> GGCAUCGAUCCGGCGAUCACCGGGGAGCCUUCGGAAGAACGGCCGGAAACGGCCCAGUAGAACCGAACGGGUUGGCCCGUCACAGCCUCAAGUCGAGCGGCCGCGCGAAAGCGUGGCAAGCGGGGUGGCAC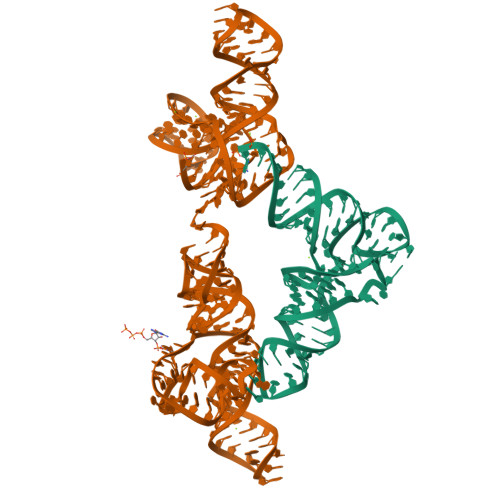CGCGGCGUUCGCGCGAAAGCGUGGCGUCGUCCCCGC;> GGGCCUAUAGCUCAGGCGGUUAGAGCGCUUCGCUGAUAACGAAGAGGUCGGAGGUUCAAGUCCUCCUAGGCCCGCCA> MTVLHWATISPFLLAILIPFLYKYARRIHTGWFVLALPLVLFIYFIRYLSVTSTGGVVEHTIPWVPSLGINFTVFVDGLSLLFALLITGIGTLVILYSIFYLSKKTESLNNFYVYLLMFMGAMLGVVLSDNLIVLYVFWELTSLASSLLISYWFHREKSTYGAQKSMLITVFGGFAMLGGFSLLYVMTGTFSIRGIIENVDLVTSSELFLPAMILVLLGAFTKSAQFPFHIWLPDAMEAPTPVSAYLHSATMVKAGIYLVARLTPVFAGSAEWFWLLTGFGVVTLLWGSTSAVRQKDLKGILAFSTVSQLGLIMTLLGLGSAAIYFGDSVDPAFYSFAIMAAIFHLINHATFKGSLFMTAGIIDHETGTRDIRKLGGLMAIMPVTFTVSLIGLASMAGLPPFNGFLSKEMFFTALLRATEMNTFNMETFGIIIVVLAWIASVFTFLYCLIMFFKTFTGKFKPENYDVKVHEAPIGMLISPVILGSLVIVFGFFPNILAYTIIEPAMQAILPTLLADGEVFYVNIYMWHGFNAELFMTMGVVAAGIILFLMMKNWAKTAFYMKERDPLNWFYDNSLSGVITGSQAVTRIQMTGLLRDYFAYMTTFMILLLGYTMFRYDAFTIDTTNVTGIAPYIWVITLVFIAATLSIPF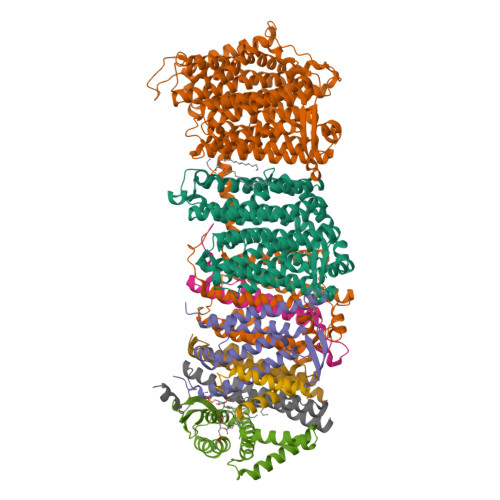INKRITAVVVVGVIGFLLALLFVVFRAPDLALTQLLVETVTVLLLMLAFYHLPELRKEEFKPRFNIVNLIISIGVGFLVTAIALSSLALGNEAGIEPISQFFVENSKELAGGYNMVNVILVDFRGLDTLLEVLVLGIAALGVIALIKLRMTGREDV;> MKNLKSNDVLLHSVTRVVTFIILAFSVYLFFAGHNNPGGGFIGGLMTASALLLMYLGFDMKSIKKAIPFDFTKMIAFGLLLAIITGFGGLLVGDPYLTQYFEYYQIPILGETELTTALPFDLGIYLVVVGIALTIILTIAEDDM;> MEILMSITVGVLFMVGTYLILTKSLLRVVVGLILLSHGAHLLLLTMAGLQRGAPPLLHLEATTYSDPLPQALILTAIVISFGVTSFLLVLAYRTYKEHKTDDLDQLRGSADE;> MNNLVILPILIPFIVGTILILFAKNHSLQRVISGFTVIGMLLVAIYLAMDVYQNGISVLELGNWQAPFGIVLVADMFATMMVILASIVGVVCLFFAFQTISSEREKYYFYPFYFFLLAGVNGAFLTGDLFNLFVFFEVMLIASYILIVLGGTKYQLRESLKYVMINVFASILFIVGVAYIYSVTGTLNMADLAVKVGQLEQTGVLNVIAVIFLVVFAMKGGLFPLYFWLPRSYYGPPAAIAALFGGLLTKVGIYAIMRTFTLIFTHDPDFTHMLILILAGLTMFFGVLGAVSQFDFKRILSYHIISQVGYMVMGLGIYTQLAIAGAIYYIAHHIIVKAALFLFAGATQRITGTTDLKKMGGLLKTHPWLAWMFFISAISLAGIPPLSGFFSKFALILAAFLNENYIIAAVALAVGLLTLFSMMKIFIYAFWGEQKHTEQQANFKVGKLLLPIVPLVALTIILGFAAEPIFQYSLQVADQILDPTIYIESVLKE;>[2x]MAFQILLNLVIAVIWVNFQNSYTAVDFLIGYVVGIFILFVLRRFLRFDFYMRRVWAIIKLIVLFFKELILANIDVIKIVLSPKMNIQPGIVAVPTKLKTDWELSLLASLISLTPGTLSMDFSDDNKYIYIHAIDVPNKEKMIRDIHDTFERAILEVTN;> MFQSILMIVLVVMSISLFVCFIRTLIGPTMSDRIVALDTFGINLIGFIGVIMMLQETLAYSEVVLVISILAFIGSIALSKFIERGVVFDRG;> MTAVEIIISIFVLIGGFLSLLGSIGIIRFPDVYGRLHAATKSATLGVISIMLATFLFFFLVHGEFVGKLLLTILFVFLTAPVAGMMMGRSAYRVGVPLWEKSTQDDLKKMYEKKMKGSNHHHHHHDYKDDDDK> LDPRLGANAFLIIRLDRIIEKLRTKLDEAEKIDPEHFVSEIDARVTKIEGTHCEKRTFQCGGNEQECISDLLVCDGHKDCHNAHDED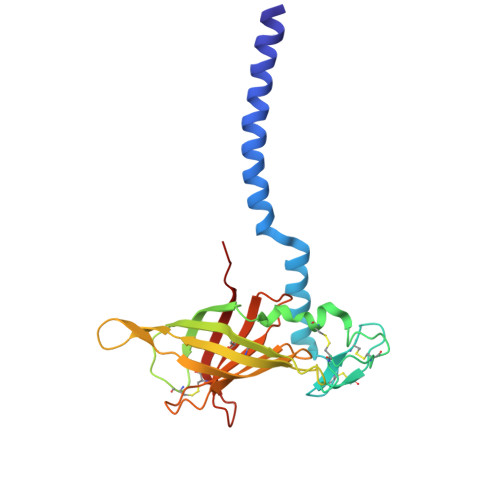PDVCDTSVVKAGNVFSGTSTWHGCLAREDHVTRITITASKRRKFFTARIWLRALVESELERHGENVTSSFNAKGYYNFASRRLILLPTDDHDDHLAVVCSFNRGDNERAECHRVTEATLHQCADLFVTLEEHD> GTTSQKHRDFVTEPMGEKPVGSLAGIGEVLGKKLEERGFDKA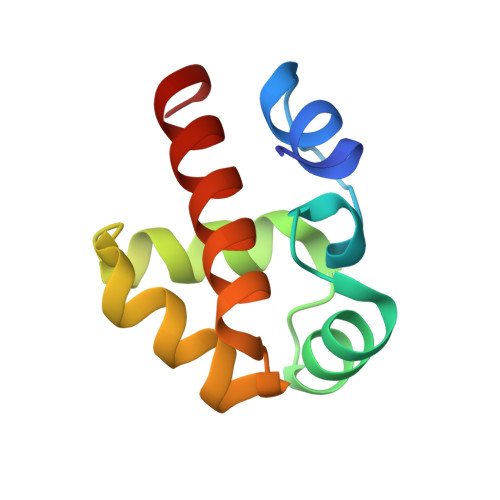YVVLGQFLVLKKDEDLFREWLKDTAGANAKQSRDAFGALREWADAFL> MSRLDKSKVINSALELLNEVGI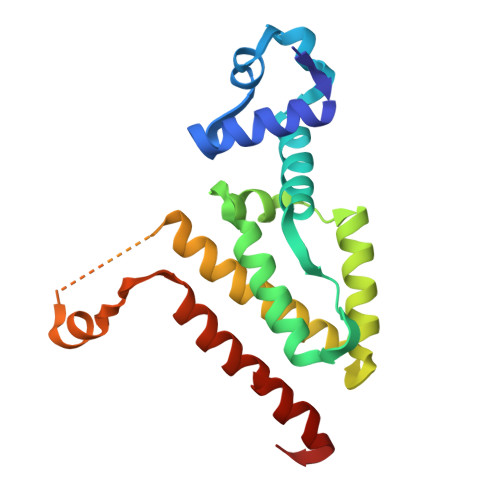EGLTTRKLAQKLGVEQPTLYWHVKNKRALLDALAVEILARHHDYSLPAAGESWQSFLRNNAMSFRRALLRYRDGAKVHLGTRPDEKQYDTVETQLRFMTENGFSLRDGLYAISWVSHFTLGAVLEQQEHTAALTDRPAAPDENLPPLLREALQIMDSDDGEQAFLHGLESIIRGIEVQLTALLQIV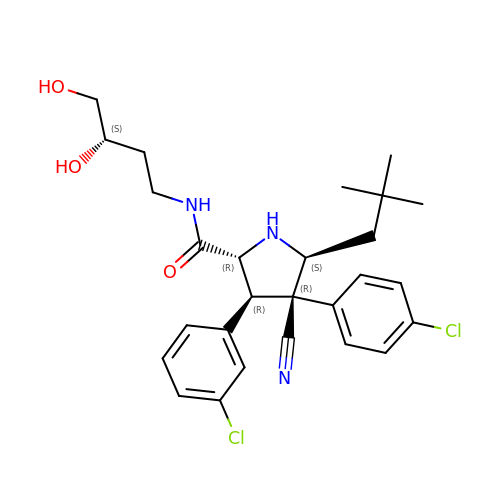(3R,4R,5S)-3-(3-chlorophenyl)-4-(4-chlorophenyl)-4-cyano-N-[(3S)-3,4-dihydroxybutyl]-5-(2,2-dimethylpropyl)-D-prolinamide | C27 H33 Cl2 N3 O3 | ZSZGGSIFAMXPIG-CPASSRBFSA-N>TVTYTNRVADARLGTFSQLLLQWKGSIYKLLYSEFLIFISLYFAISLVYRLILSESQRLMFEKLALYCNSYAELIPVSFVLGFYVSLVVSRWWAQYESIPWPDRIMNLVSCNVDGEDEYGRLLRRTLMRYSNLCSVLILRSVSTAVYKRFPSMEHVVRAGLMTPEEHKKFESLNSPHNKFWIPCVWFSNLAVKARNEGRIRDSVLLQGILNELNTLRSQCGRLYGYDWISIPLVYTQVVTVAVYSFFLACLIGRQFLDPEKAYPGHELDLFVPVFTFLQFFFYAGWLKVAEQLINPFGEDDDDFETNWLIDRNLQVSLMAVDEMHQDLPILEKDLYWNEPDPQEGEEF[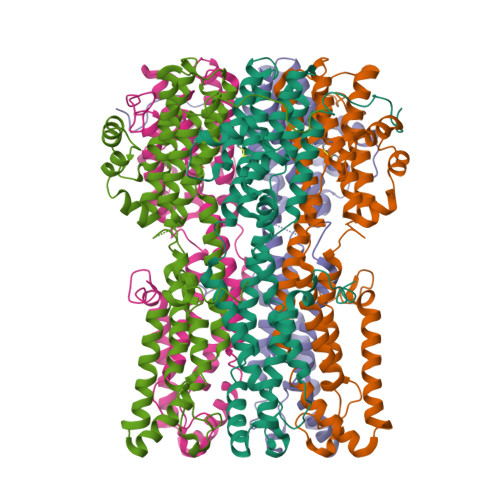5x]Here, we report the cryo-EM structure of the cyanophage P-SCSP1u, a representative member of the MPP-C phages, in its native form at near-atomic resolution, which reveals the assembly mechanism of the capsid and molecular interaction of the portal-tail complex. Overall, the P-SCSP1u virion possesses an icosahedral capsid with a diameter of ~600 Å and a short tail of ~190 Å in length. The recently identified MPP-C (Marine Picocyanobacteria Podovirus clade C) cyanophages, belonging to the T7-like podoviruses, contain the smallest genomes among cyanopodoviruses and exhibit distinct infection kinetics. By using single-particle cryo-EM, we finally determined the structure of P-SCSP1u in its native state at 3.2 Å and 3.8 Å for the capsid and portal-tail complex, respectively.

By using sub-particle and symmetry expansion in the data processing, the resolution of capsid protein (gp19, 328 aa) has been improved to 3.2 Å, enabling the de novo model building covering nearly all residues (Ala2 to Ser328) unambiguously. The whole capsid of P-SCSP1u is solely composed of 415 copies of major capsid protein (gp19), exhibiting 60 hexameric capsomeres (hexons) and 11 pentameric capsomeres (pentons). Similar to T7 and the MPP-B cyanophage P-SSP7, P-SCSP1u does not have decoration (cement) proteins in the icosahedral capsid. As observed in T7 and two cyanopodoviruses (P-SSP7 and Syn5), each asymmetric unit of the P-SCSP1u capsid consists of one hexon and one subunit of penton, yielding a triangulation (T) number of 7 for P-SCSP1u. Each capsid protein of P-SCSP1u contains four distinct domains from N to C terminus: an extended N terminus (N-arm), a long-extended loop (E-loop), a triangular domain (A-domain) and an elongated protrusion domain (P-domain). Although sharing low sequence similarity with the major capsid protein (gp5, 385 aa) of the bacteriophage HK97, the P-SCSP1u capsid protein gp19 presents the HK97-like fold, which was first determined in phage HK9735 and has been discovered in many tailed phages and herpesviruses. The pentons and hexons are assembled by similar intra-capsomeric interactions, with A-domains constituting the core of capsomers and E-loops wrapping around the adjacent N-arms and P-domains, forming a circulating interaction mode to stabilize the capsomer. The inter-capsomeric interactions are mediated by mutual penetration of the E-loops and P-domains of neighboring capsomers and further reinforced by the extended N-arms interacting with multiple subunits to fasten the adjacent capsomers. Overall, the capsid of P-SCSP1u is assembled via non-covalent interactions to maintain the high internal pressure for DNA packaging. Consistently, the Dali Z-scores revealed that seven capsid protein subunits in the viral asymmetric unit of P-SCSP1u show higher similarities with those of T7. These structural analyses suggest that the capsid of P-SCSP1u is structurally closer to that of T7, rather than two cyanopodoviruses Syn5 and P-SSP7.

>[7x]MANFTPSRLGLVNNTGTGVKDLFLKTFAGEVLSAFRKATIFEDLHTVRTISSGKSAQFPIVGLSSTSYHSPGTQLTGNAIKHAEAVINIDDKLVSNVFIADVDEAMNHYDVRSQYSVQMGNALAYTFDQNVAAMIAQAARTSTNPNTDLPGGTRIKILKSGTANTAAAVAAVTGTDLATALFSAAEQMDINNLPEEDRYCAIDPTNYYKLVQNTTVINRDFGGRGAYAEGEVLKVAGIHIVKSNHLPKTNRSAATGENNTYHANYTDNIGLVFNKQAVGTVKLMDLKMEQTGADIHALYQGTFMVGSMMHGSGVLRPDCAIELYAANS(4-fluorophenyl)(pyridin-4-yl)methanone 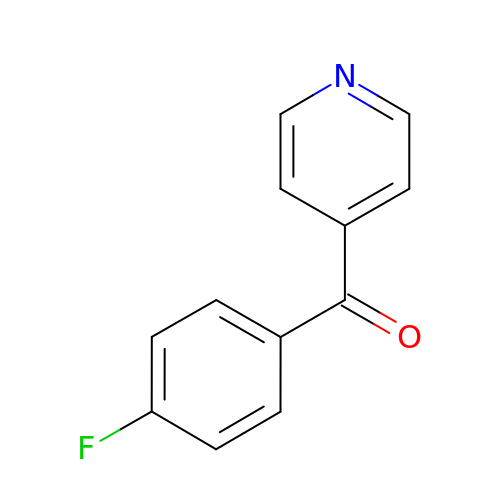| C12 H8 F N O | WTRWBYGUMQEFFI-UHFFFAOYSA-N> MMRGIDSRHELDPTLLLRDTRTFTQRLADFFADPTNISIVLISLAAVSYYFSEAATFLLIMGGIFFLYSYTRKQKLPFRLPQISRAKDYNDLKPGINKPNIARGITFFGNDRKTGEELWFANDDMRTHALIFGSTGSGKTETLVSLSYNALVQGSGFIYVDGKGDNSLYAKVFSMVRSMGREDDLLLINFMTGARDIVGPQEKRLSNTLNPFCQGSSSMLTQLVVSLMGSSGQSSDGDMWKGRAIAFVEALMRLLVYMRDEGAILLDANTIRNYFDLQRLESIVIDKVFPRDDQESVNIETIPKLVTDPLRNYLNTLPGYNKEKKGKQVSQVLEQHGFITMQLVRSFSSLADTYGHIIRTNLAEVDFKDVVLNRRILVVLLPALEKSPDELSNLGKIIVSSLKAMMAAGLGEEVEGDYRDVILRKPTNAPTPYMCILDEYGYYAVQGFAVVPAQARSLGFSAIFAGQDLPAFQKASKEEAASIGANTNIKICMKLEDPTETWDFFTKTAGEAYVTKVDSFQTKETSIANSYMDTKSSSFEKRARVDLLDLKEQTEGEAHIFFKSKIVRARMFYANPKPVKQLKINQFLKVEPPPDDYLMKLQKQLASFQSILESGDLSINKAVENEEITLISKALKESTIVEPIERGVAALIAFHGQNEPEPVEDIVEEEVEGALTIFSKLRIDPNAPPILVADKEVFSEPLLPINETRNQMITIERLAGAKDKYAGTVANELIKDFQIATSYP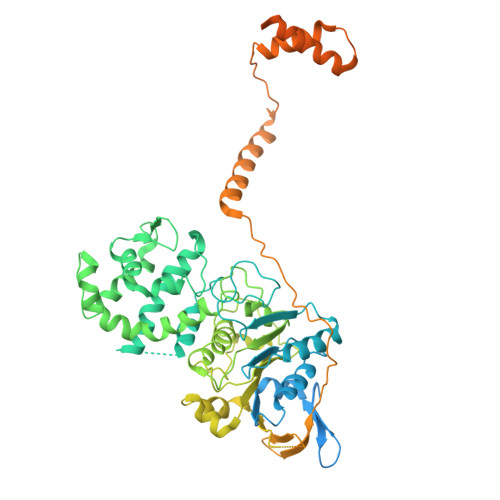PEERDVIDVQELTGIIRDLSAKISAEREKANKKAAEELT>[4x]MLGSSSLSIRTTDDKSLFARTMDFTMEPDSKVIIVPRNYGIRLLEKENVVINNSYAFVGMGSTDITSPVLYDGVNEKGLMGAMLYYATFATYADEPKKGTRGINPVYVISQVLGNCVTVDDVIEKLTSYTLLNEANIILGFAPPLHYTFTDASGESIVIEPDKTGITIHRKTIGVMTNSPGYEWHQTNLRAYIGVTPNPPQDIMMGD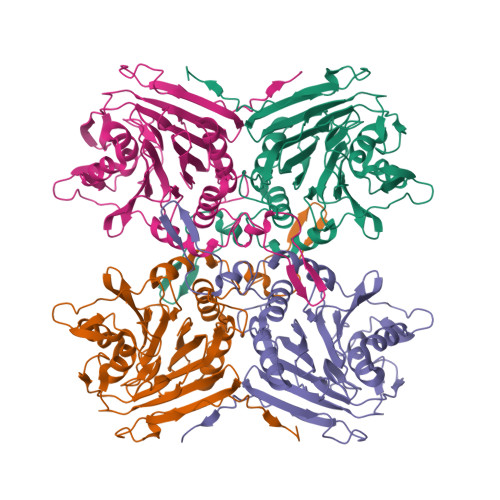LDLTPFGQGAGGLGLPGDFTPSARFLRVAYWKKYTEKAKNETEGVTNLFHILSSVNIPKGVVLTNEGKTDYTIYTSAMCAQSKNYYFKLYDNSRISAVSLMAENLNSQDLITFEWDRKQDIKQLNQVNVMS> MSKIFVNPSAIRAGLADLEMAEETVDLINRNIEDNQAHLQGEPIEVDELPEDENLYFQGMDADRIVFRSNNQVVSLRPEIIADQYEYKYPAIKDLKKPCITLGKAPDLNKAYKSVLSGMNAAKLDPDDVCSYLAAAMQFFEGTCPEDWTSYGILIARKGDKITPNSLVEIKRNDVEGNWALTGGMEMTRDPTVSEHASLVGLLLSLYRLSKISGQNTGNYKTNIADRIEQIFETAPFVKIVEHHTLMTTHKMCANWSTIPNFRFLAG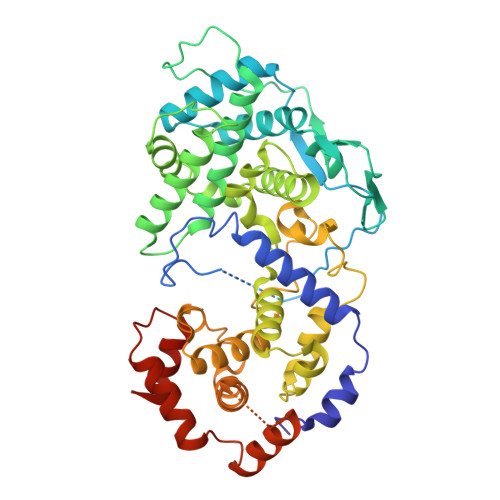TYDMFFSRIEHLYSAIRVGTVVTAYEDCSGLVSFTGFIKQINLTAREAILYFFHKNFEEEIRRMFEPGQETAVPHSYFIHFRSLGLSGKSPYSSNAVGHVFNLIHFVGCYMGQIRSLNATVIAACAPHEMSVLGGYLGEEFFGRGTFERRFFRDEKELQEYEAAELTKTDVALADDGTVDEDDEDYFSGEARGPEAVYARIMMNGGRLKRSHIRRYVSVSSNHQARPNSFAEFLNKTYSSDSHHHHHHHH> AERPTLPIPDLL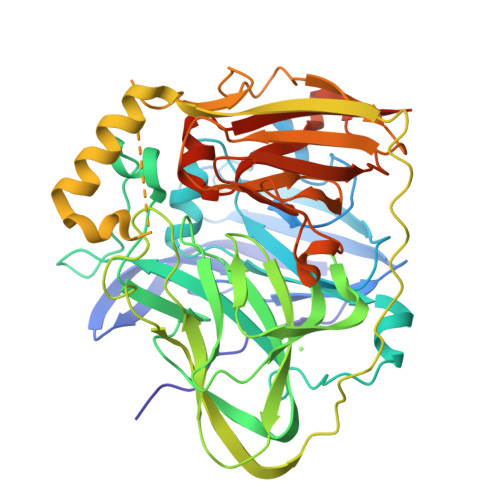TTDARNRIQLTIGAGQSTFGGKTATTWGYNGNLLGPAVKLQRGKAVTVDIYNQLTEETTLHWHGLEVPGEVDGGPQGIIPPGGKRSVTLNVDQPAATCWFHPHQHGKTGRQVAMGLAGLVVIEDDEILKLMLPKQWGIDDVPVIVQDKKFSADGQIDYQLDVMTAAVGWFGDTLLTNGAIYPQHAAPRGWLRLRLLNGCNARSLNFATSDNRPLYVIASDGGLLPEPVKVSELPVLMGERFEVLVEVNDNKPFDLVTLPVSQMGMAIAPFDKPHPVMRIQPIAISASGALPDTLSSLPALPSLEGLTVRKLQLSMDPILDMMGMQMLMEKYGDQAMAGMDHSQMPRFMDYWEGLNMNHGGKFDFHHANKINGQAFDMNKPMFAAAKGQYERWVISGVGDMMLHPFHIHGTQFRILSENGKPPAAHRAGWKDTVKVEGNVSEVLVKFNHDAPKEHAYMAHCHLLEHEDTGMMLGFTVKDPNSSSVDKLAAALEHHHHHH> MDPAHHIKDTSAELLSQQDFSILQSRLLEFLASQ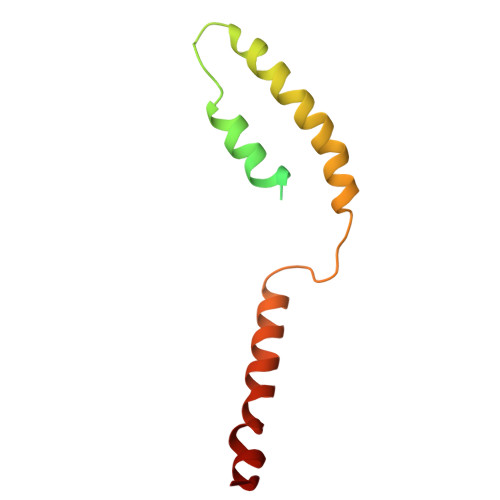EARETVTASKELTLLRQGIRQLKEKVSKMEPEEMTVKEKKSIIEILKARIALKKAFLKMALSESNDTVVKKEDVRESPVDTFMENAT> MQRYYFTVHFLPKQANLALLTGRCISIMHGFILKHNIEGMGVTFPAWSDSSIGNEIAFVYTDKEILNTLKDQAYFVDMQDCGFFKVSQVLAVPDSCEEVRFIRNQAVAKIFTGESRRRLKRLQKRALARGEDFNPKKIEAPR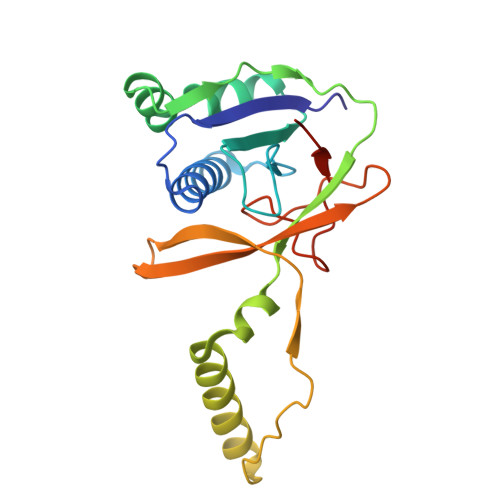EIDIFHRVAMTSKSSQEDYILHIQKQDVDCQAEPYFSNYGLASNEKFKGTVPDLSPSIDRN> MERTFTPNVMQPTPLLPTTNDGRVTFGEAFNDLKDLARRYQLYWEGTILEGNLRAIRRNSALVQLPLY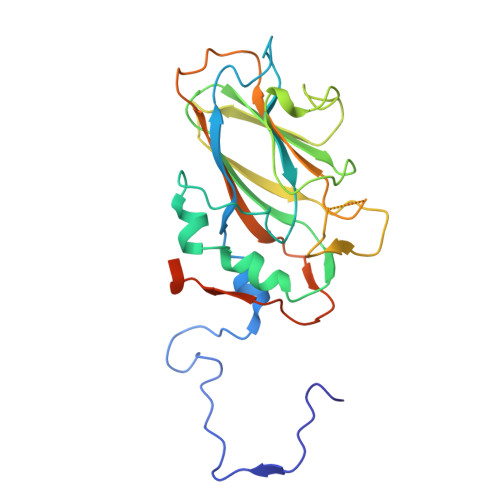PHGLRIQPDVNNPIWNIMRDGHIPVISSGFRYFRGGLRLRIVVEGLNSCVWVQHHPDRPSIFSRPIIGRYIAAKDAYRNHAYAAYVQNMSVNRTIEVEVPFYQPGLYGMLNASDNNTANSFDRLRFTGLGDLLIGIEGEQPIPKEGIEISVYYSIADDFSFNIFCGFPPMVYCDETYSAATPDLAQYFEDEVTIAQPE>[4x]MTADELVFFVNGKKVVEKNADPETTLLAYLRRKLGLRGTKLGCGEGGCGACTVMLSKYDRLQDKIIHFSANACLAPICTLHHVAVTTVEGIGSTKTRLHPVQERIAKSHGSQCGFCTPGIVMSMYTLLRNQPEPTVEEIEDAFQGNLCRCTGYRPILQGFRTFAK;>PKQLRFEGERVTWIQASTLKELLDLKAQHPEAKLVVGNTEIGIEMKFKNQLFPMIICPAWIPELNAVEHGPEGISFGAACALSSVEKTLLEAVAKLPTQKTEVFRGVLEQLRWFAGKQVKSVASLGGNIITASPISDLNPVFMASGTKLTIVSRGTRRTVPMDHTFFPSYRKTLLGPEEILLSIEIPYSREDEFFSAFKQASRREDDIAKVTCGMRVLFQPGSMQVKELALCYGGMADRTISALKTTQKQLSKFWNEKLLQDVCAGLAEELSLSPDAPGGMIEFRRTLTLSFFFKFYLTVLKKLG[4x];>DTVGRPLPHLAAAMQASGEAVYCDDIPRYENELFLRLVTSTRAHAKIKSIDVSEAQKVPGFVCFLSADDIPGSNETGLFNDETVFAKDTVTCVGHIIGAVVADTPEHAERAAHVVKVTYEDLPAIITIEDA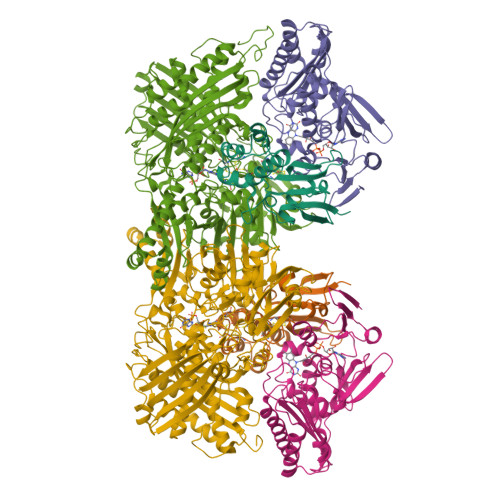IKNNSFYGSELKIEKGDLKKGFSEADNVVSGELYIGGQDHFYLETHCTIAIPKGEEGEMELFVSTQNAMKTQSFVAKMLGVPVNRILVRVKRMGGGFGGKETRSTLVSVAVALAAYKTGHPVRCMLDRNEDMLITGGRHPFLARYKVGFMKTGTIVALEVDHYSNAGNSRDLSHSIMERALFHMDNCYKIPNIRGTGRLCKTNLSSNTAFRGFGGPQALFIAENWMSEVAVTCGLPAEEVRWKNMYKEGDLTHFNQRLEGFSVPRCWDECLKSSQYYARKSEVDKFNKENCWKKRGLCIIPTKFGISFTVPFLNQAGALIHVYTDGSVLVSHGGTEMGQGLHTKMVQVASKALKIPISKIYISETSTNTVPNSSPTAASVSTDIYGQAVYEACQTILKRLEPFKKKNPDGSWEDWVMAAYQDRVSLSTTGFYRTPNLGYSFETNSGNAFHYFTYGVACSEVEIDCLTGDHKNLRTDIVMDVGSSLNPAIDIGQVEGAFVQGLGLFTLEELHYSPEGSLHTRGPSTYKIPAFGSIPTEFRVSLLRDCPNKKAIYASKAVGEPPLFLGASVFFAIKDAIRAARAQHTNNNTKELFRLDSPATPEKIRNACVDKFTTLCVTGAPGNCKPWSLRV[4x]> SSSKFQQVEQDVKAIEVSLSARIGVSVLDTQNGEYWDYNGNQRFPLTSTFKTIACAKLLYDAEQGKVNPNSTVEIKKADLVTYSPVIEKQVGQAITLDDACFATMTTSDNTAANIILSAVGGPKGVTDFLRQIGDKETRLDRIEPDLNEGKLGDLRDTTTPKAIASTLNK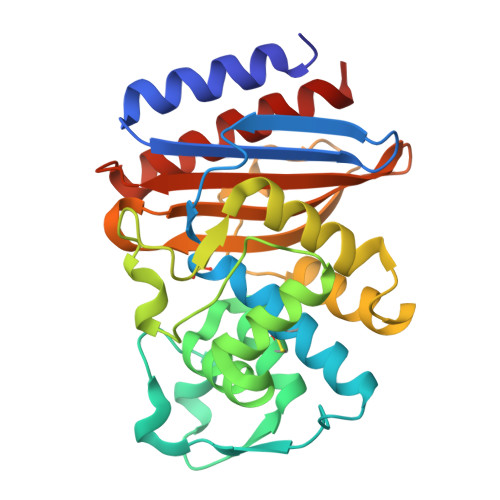FLFGSALSEMNQKKLESWMVNNQVTGNLLRSVLPAGWNIADKSGAGGFGARSITAVVWSEHQAPIIVSIYLAQTQASMEERNDAIVKIGHSIFDVYTSQSR> GPHMLEMKIFSESHKTVFVVDH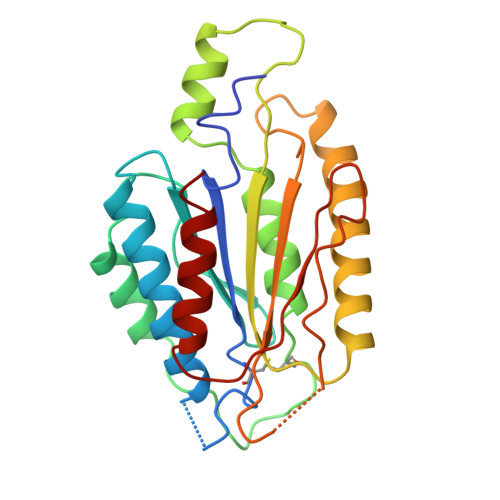CPYMAESCRQHSKSLWTCSVESSMEYCRIMYDIFPFKKLVNFIVSDSGAHVLNSWTQEDQNLQELMAALAAVGPPNPRADPECCSILHGLVAAVETLCKITEYQHEARTLLMENAERVGNRGRIICITNAKSDSHVRMLEDCVQETIHEHNKLAANSDHLMQIQKCELVLIHTYPVGEDSLVSDRSKKELSPVLTSEVHSVRAGRHLATKLNILVQQHFD>GAMGSMSKSLKKLVEESREKNQPEVDMSDRGISNMLDVNGLFTLSHITQLVLSHNKLTMVPPNIAELKNLEVLNFFNNQIEELPTQISSLQKLKHLNLGMNRLNTLPRGFGSLPALEVLDLTYNNLSENSLPGNFFYLTTLRALYLSDNDFEILPPDIGKLTKLQILSLRDNDLISLPKEIGELTQLKELHIQGNRLTVLPPELGNLDLTGQKQVFKAENNPWVTPIADQFQLGVSHVFEYIRSETYKYLYGRHMQANPEPPKKNNDKSKKISRKPLAAKNR[2x];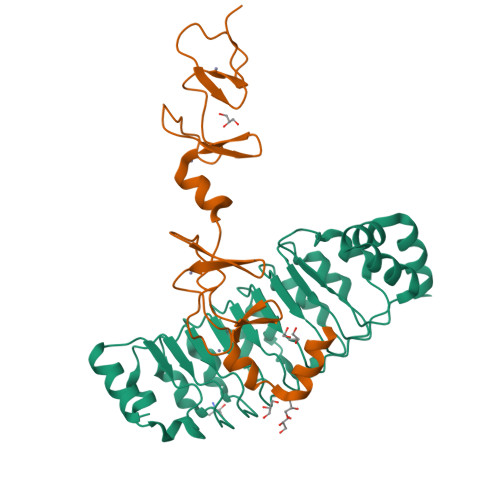>GPGSMGVPICGACRRPIEGRVVNAMGKQWHVEHFVCAKCEKPFLGHRHYERKGLAYCETHYNQLFGDVCFHCNRVIEGDVVSALNKAWCVNCFACSTCNTKLTLKNKFVEFDMKPVCKKCYEKFPLELKKRLKKLAETLGRK[2x]> SNAMWETKFAKEGLTFDDVLLVPAKSDVLPNDVDLSVEMAPSLKLNVPIWSAGMDTITEAKMAIAIARQGGIGVVHKNMSIEQQAEEIEKVKRSGGLLAAAAVGITNDTFVRVEKLIEAGVDAIVIDTAHGHSAGVINKISEIRQTFKDVVIVAGNVATAEGARALFEVGVDIVKVGIGPGSICTTRVVAGVGVPQITAIYDCATVAREFGKTIIADGGIKYSGDIVKALAAGGNAVMLGSMLAGTDESPGETEIFQGRQFKTYRGMGSLAAMEHGSKDRYFQADAKKLVPEGIEG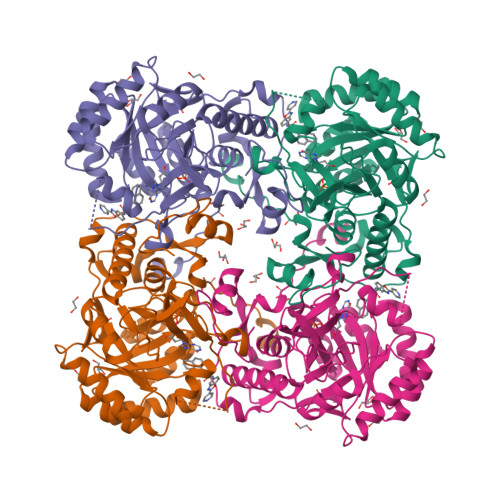RVPYKGSVADIIFQLVGGIRSGMGYTGSPDLRHLREEAAFVRMTGAGLRESHPHDIQITKEAPNYSIS Plant HISN5 catalyzes the sixth step of the HBP, in which imidazole-glycerol phosphate (IGP) is dehydrated to form imidazole-acetol phosphate (IAP). The MtHISN5 subunit contains a four α-helix bundle sandwiched between two β-sheets whose four strands are almost perpendicular to each other. In solution, MtHISN5 forms a homo 24-mer with octahedral (432) symmetry of approx. 110 Å diameter and a total mass of 540 kDa. The dimensions of the MtHISN5 oligomer did not change significantly after the binding of IG2, indicating a lack of major conformational rearrangements. The active site of MtHISN5 (see below) contains two Mn2+ cations (Mn1 and Mn2) bound by residues belonging to different subunits.

The crystal structures cover the MtHISN5 sequence starting from Gly77 or Ala78 through Arg260/261 (chain and structure-dependent). Both cryoEM structures (unliganded and IG2 complex) have been reconstructed from EM maps with octahedral symmetry, and therefore contain 24 identical protein chains, spanning from Ala78 to Arg261 (IG2 complex) and Arg262 (unliganded). The cryoEM MtHISN5-IG2 complex structure reveals detailed information about the most likely substrate positioning before catalysis. The imidazole ring is trapped between manganese ions, facing its Nδ towards Mn2 and Nϵ towards Mn1. While the formation of the active site with the bi-Mn2+ cluster requires a contribution of residues from two subunits, a third subunit participates in substrate/product binding by contributing guanidines of Arg167** and Arg189** that bind the phosphate group. However, based on our complex with IG2, these polar H-bonds are rather weak, with the donor-acceptor distances of 3.5 – 3.8 Å. It must be emphasized that our MtHISN5-IG2 complex structure is a spectacular example where the cryoEM maps are of such a high quality that they permit resolving stereoisomers of ligands bound to a protein. In fact, we expected the reaction product, IAP as the enzyme was incubated with cIGP (at 2 mM concentration) for 2 days prior to the cryoEM grid preparation. We clearly recognized IG2 based on EM maps (inset). Interestingly, with 2 mM cIGP, the initial lag reached the maximum time that the PEAQ-ITC apparatus offers (170 min). This peculiar behavior can likely be attributed to the contamination of cIGP with IG2, as revealed by our cryoEM experiments.

>[24x]PTFPIDSGARIGEMKRVTKETNVSVKINLDGTGVADNSSGIPFLDHMLDQLASHGLFDVHVKATGDTHIDDHHTNEDVALAIGTALLQALGDRKGINRFGNFSAPLDEALVHVSLDLSGRPHLGYDLNIPTQRVGKYDTQLVEHFFQSLVNTSGMTLHIRQFSGTNSHHIIEATFKAFARALRQATEYDTRRRGTIPSSKGVLSRS> SNWVMQEENKQGNLTPLFEELLQQCPPGGQNKTAHMVSAYQLAQGNWMPTSCHVFMGTISARRTKTHPYEAYVKLRELVEEHKMKTLCPGSSLGKHN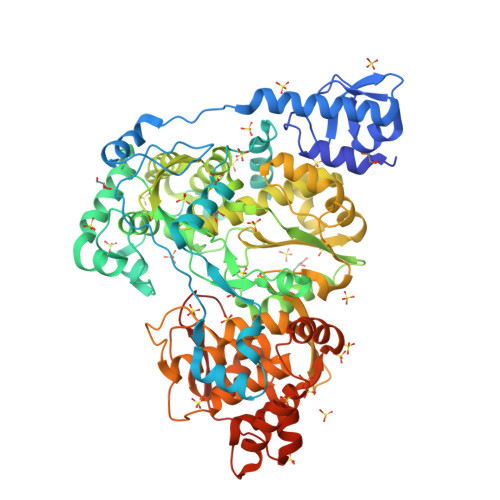EWIIGKIKYQGNLRTKHMLNPGKVAEQLCREGHRHNVYNKTIGSVMTATGIRLEKLPVVRAQTDTTNFHQAIRDKIDKEENLQTPGLHKKLMEVFNALKRPELESSYDAVEWEELERGINRKGAAGFFERKNIGEILDSEKNKVEEIIDNLKKGRNIKYYETAIPKNEKRDVNDDWTAGDFVEEKKPRVIQYPEAKTRLAITKVMYKWVKQKPVVIPGYEGKTPLFQIFDKVKKEWDQFQNPVAVSFDTKAWDTQVTTKDLELIKDIQKYYFKKKWHKFIDTLTMHMSEVPVISADGEVYIRKGQRGSGQPDTSAGNSMLNVLTMIYAFCEATGVPYKSFDRVAKIHVCGDDGFLITERALGEKFASKGVQILYEAGKPQKITEGDKMKVAYQFDDIEFCSHTPIQVRWSDNTSSYMPGRNTTTILAKMATRLDSSGERGTIAYEKAVAFSFLLMYSWNPLIRRICLLVLSTELQVKPGKSTTYYYEGDPISAYKEVIGHNLFDLKRTSFEKLAKLNLSMSVLGAWTRHTSKRLLQDCVNVGVKEGNWLVNADRLVSSKTGNRYIPGEGHTLQGRHYEELVLARKQINNFQGTDRYNK Utilizing the published genome sequence of the organism, we hypothesized that the genes 0612, 0638, and 0637 encode for a 4,6-dehydratase, an aminotransferase, and an N-acetyltransferase, respectively, which would be required for the biosynthesis of one of the diacetamido-sugars, 2,4-diacetamido-2,4,6-trideoxy-d-glucose, starting from UDP-N-acetylglucosamine. In this report we present functional and structural data that demonstrate the proteins encoded by the 0638 and 0637 genes do indeed correspond to an aminotransferase (hereafter referred to as Pcryo_0638) and an N-acetyltransferase (Pcryo_0637). In summary, we have demonstrated that the genes in P. cryohalolentis, namely 0638 and 0637, encode for a PLP-dependent aminotransferase and an N-acetyltransferase, respectively. The data presented herein confirm the hypothesized functions of these enzymes and provide new insight into an unusual sugar biosynthetic pathway in Gram-negative bacteria.

The crystals utilized for the investigation belonged to the space group R3 with one subunit in the asymmetric unit. The N-acetyltransferases belonging to the left-handed β-helix superfamily are known to function as trimers, and thus the local threefold rotational axis of Pcryo_0637 packed along a crystallographic triad. The overall architecture of the subunit is distinctly bilobal with an N-terminal domain delineated from Ser 2 to Ser 93 and the C-terminal domain formed by Leu 94 to Ala 218. The N-terminal domain, characterized by a five-stranded mixed β-sheet surrounded by three α-helices, provides a binding platform for the UDP molecule. The C-terminal domain displays a classical left-handed β-helix motif with six complete turns. As can be seen, the acetyl-CoA ligand adopts an extended conformation, which allows the placement of the acetyl group into the active site region that is located at the interface of the two domains. The acetyl-CoA moieties are wedged between the subunits of the trimer. There is one cis-peptide bond between Asn 212 and Pro 213.

> MSKVFAVYGASGCGRSLMPVANEQLRILEGDTDSQIVFIDDALDDNITVNGYTAMNYTKFKSIKNDDKFVLIAIANSSIRQKIADKLVKDGISLWTVQGMTTLIMDEVSIDAGAALSPFVTIAANVTIGKCFHANLYSYVEHDCIIGDYVTFAPRVSCNGNIHIHDHAYIGTGAVIKQGTPDKPLIIGKGAIVGMGAVVTKEVPAGAVVIGNPARLLNKLEHHHHHH>MASEKPLAAVTCTAPVNIAVIKYWGKRDEELVLPINSSLSVTLHQDQLKTTTTAVISKDFTEDRIWLNGREEDVGQPRLQACLREIRCLARKRRNSRDGDPLPSSLSCKVHVASVNNFPTAAGLASSAAGYACLAYTLARVY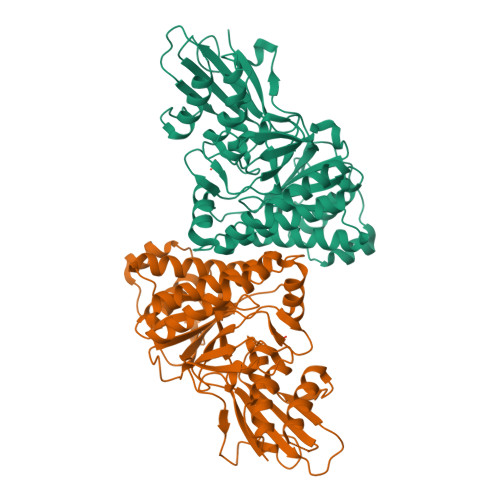GVESDLSEVARRGSGSACRSLYGGFVEWQMGEQADGKDSIARQVAPESHWPELRVLILVVSAEKKLTGSTVGMRASVETSPLLRFRAESVVPARMAEMARCIRERDFPSFAQLTMKDSNQFHATCLDTFPPISYLNAISWRIIHLVHRFNAHHGDTKVAYTFDAGPNAVIFTLDDTVAEFVAAVWHGFPPGSNGDTFLKGLQVRPAPLSAELQAALAMEPTPGGVKYIIVTQVGPGPQILDDPCAHLLGPDGLPKPAA[2x]>GSHMTKKGKTLMMFVTVSGNPTEKETEEITSLWQGSLFNANYDVQRFIVGSDRAIFMLRDGSYAWEIKDFLVSQDRCAEVTLE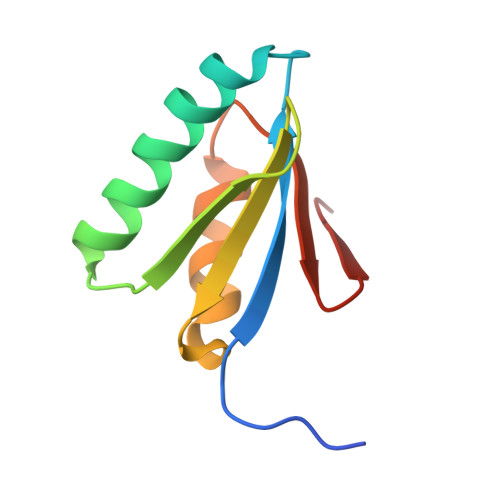GQMYPG[2x]3,4-DI-1H-INDOL-3-YL-1H-PYRROLE-2,5-DICARBOXYLIC ACID | C22 H15 N3 O4 | 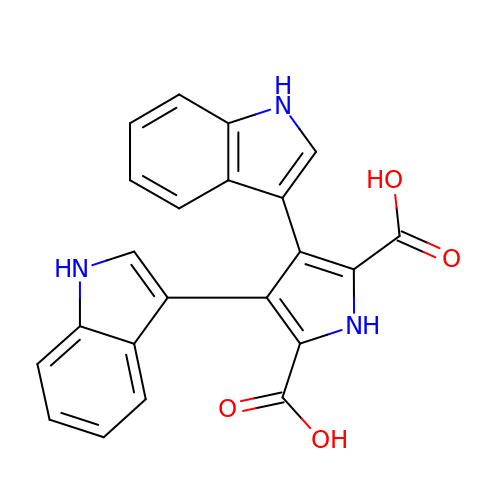FZDVNXHYGMEEDT-UHFFFAOYSA-N> HHAADYVLYKDATKPVEDRVADLLGRMTLAEKIGQMTQIERLVATPDVLRDNFIGSLLSGGGSVPRKGATAKEWQDMVDGFQKACMSTRLGIPMIYGIDAVHGQNNVYGATIFPHNVGLGATRDPYLVKRIGEATALEVRATGIQYAFAPCIAVCRDPRWGRCYESYSEDRRIVQSMTELIPGLQGDVPKDFTSGMPFVAGKNKVAACAKHFVGDGGTVDGINENNTIINREGLMNIHMPAYKNAMDKGVSTVMISYSSWNGVKMHANQDLVTGYLKDTLKFKGFVISDWEGIDRITTPAGSDYSYSVKASILAGLDMIMVPNKYQQFISILTGHVNGGVIPMSRIDDAVTRILRVKFTMGLFENPYADPAMAEQLGKQEHRDLAREAARKSLVLLKNGKTSTDAPLLPLPKKAPKILVAGSHADNLGYQCGGWTIEAQGDTGRTTVGTTILEAVKAAVDPSTVVVFAENPDAEFVKSGGFSYAIVAVGEHPYTETKGDNLNLTIPEPGLSTVQAVCG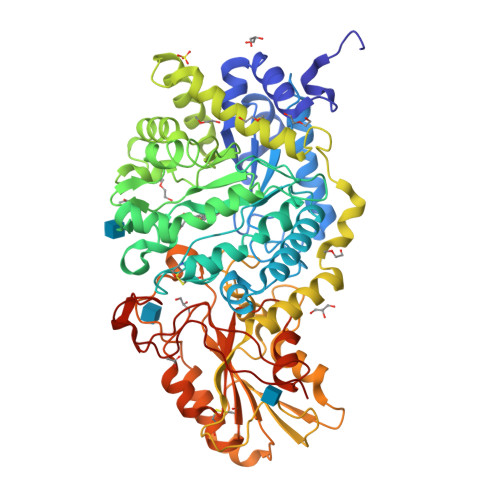GVRCATVLISGRPVVVQPLLAASDALVAAWLPGSEGQGVTDALFGDFGFTGRLPRTWFKSVDQLPMNVGDAHYDPLFRLGYGLTTNATKKY>MCTGLRFTDDQGNLYFGRNLDVGQDYGEGVIITPRNYPLPYKFLDNTTTKKAVIGMGIVVDGYPSYFDCFNEDGLGIAGLNFPHFAKFSDGPIDGKINLASYEIMLWVTQNFTKVSDVKEALKNVNLVNEAINSSFAVAPLHWIISDKDEAIIVEVSKQYGMKVFDDKLGVLTNSPDFNWHLTNLGNYTGLDPHDATAQSWNGQKVAPWGVGTGSLGLP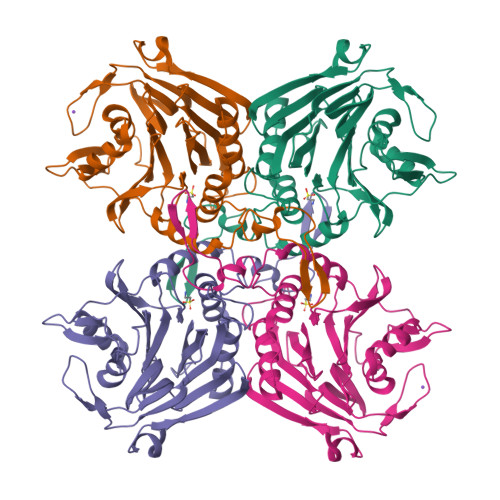GDSIPADRFVKAAYLNVNYPTVKGEKANVAKFFNILKSVAMIKGSVVNKLGSDEYTVYTACYSAATKTYYCNFENDFELKTYKLDDETMNADKLITYHHHHHH[4x]> ALANTFLVKEDSKNVTAYTPFATPITDSKSDLVSLAQLDSSYQIADQTIHNTNLFVLFKSRDVKVKYESSGSNNISFDSTSQGEKPSYVVEFTNSTNIGIKWTMVKKYQLDVPNVSSDMNQVLKNLILEQPLTKYTLNSSLAKEKGKTQREVHLGSGQANQWTSQRNQHDLNNNPSPNASTGFKLTTGNAYRKLSESWPIYEPIDGTKQGKGKDSSGWSSTEENEAKNDAPSVSGGGSSSGTFNKYLNTKQALESIGILFDDQTPRNVITQLYYASTSKLAVTNNHIVVMGNSFLPSMWYWVVERSAQENASNKPTWFANTNLDWGEDKQKQFVENQLGYKETTSTNSHNFHSK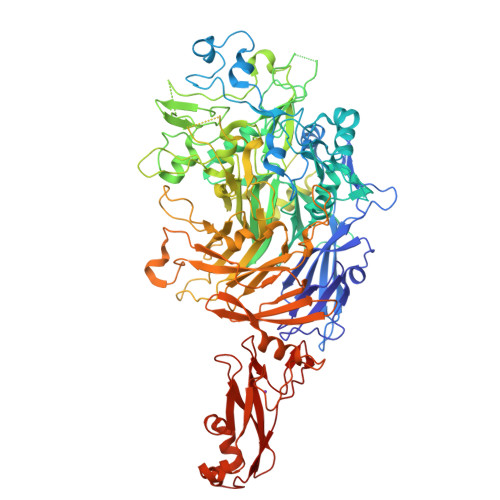SFTQPAYLISGIDSVNDQIIFSGFKAGSVGYDSSSSSSSSSSSSTKDQALAWSTTTSLDSKTGYKDLVTNDTGLNGPINGSFSIQDTFSFVVPYSGNHTNNGTTGPIKTAYPVKKDQKSTVKINSLINATPLNSYGDEGIGVFDALGLNYNFKSNQERLPSRTDQIFVYGIVSPNELRSAKSSADSTGSDTKVNWSNTQSRYLPVPYNYSEGIIDADGFKRPENRGASVTTFSGLKSIAPDGFANSIANFSVGLKAGIDPNPVMSGKKANYGAVVLTRGGVVRLNFNPGNDSLLSTTDNNIAPISFSFTPFTAAESAVDLTTFKEVTYNQESGLWSYIFDSSLKPSHDGKQTPVTDNMGFSVITVSRTGIELNQDQATTTLDVAPSALAVQSGIQSTTQTLTGVLPLSEEFSAVIAKDSDQNKIDIYKNNNGLFEIDTQLSNSVATNNGGLAPSATENRVDAWGKVEFADNSVLQARNLVDKTVDEIINTPEILNSFFRFTPAFEDQKATLVATKQSDTSLSVSPRIQFLDGNFYDLNSTIAGVPLNIGFPSRVFAGFAALPAHHHHHH1-{1-[2-(methylsulfonyl)phenyl]-7-phenoxyindolizin-3-yl}ethanone | C23 H19 N O4 S | 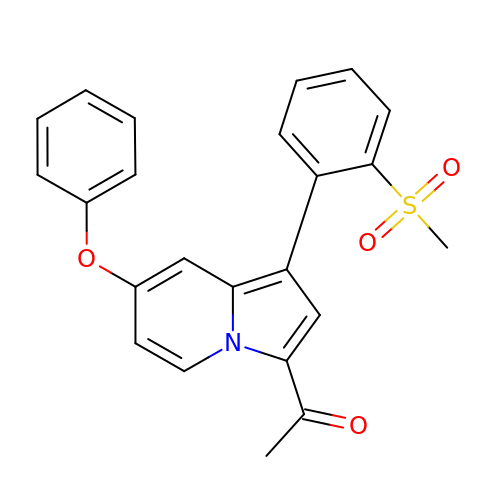DNOOBVIUDXIJGO-UHFFFAOYSA-N>GAMGSSSVWGVAFSPDGQTIASASDDKTVKLWNRNGQLLQT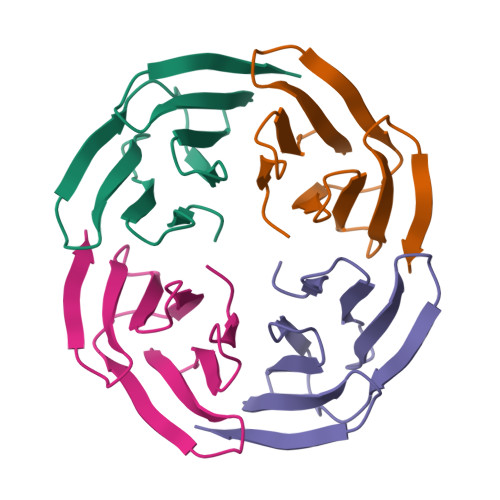LTGHSSSVWGVAFSPDGQTIASASDDKTVKLWNRNGQLLQTLTGH[4x]1,1,1,3,3,3-hexafluoropropan-2-yl 3-(3-phenyl-1,2,4-oxadiazol-5-yl)azetidine-1-carboxylate | C15 H11 F6 N3 O3 | 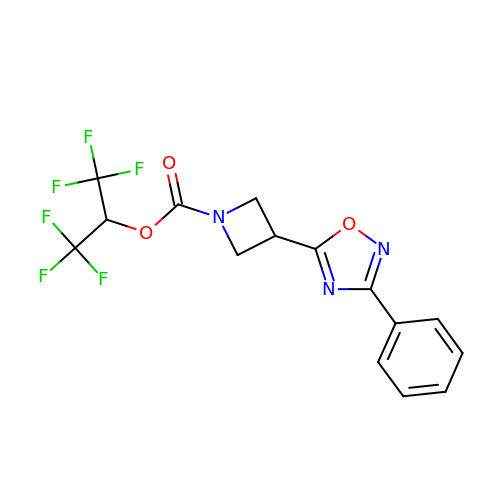MQSOFDLFKHBDFY-UHFFFAOYSA-N>[4x]MAPTNESPKHAETRIVTDAPRNSESVGDHLFNGGVNHHDEDPDAYTKMYGPLVGYDPRNPTTLFANARQTGTQLVAPRKAREILTGIYSFEPTVLAFQREFVKRANAVAQPDLNSDGFSLNGLHTTFDSIRSVSGYPQWPVSALPKSNVGLLRDLKLQERMTARQVVIAREIWKRVWGHMKPTAIKIPKMSTSGPPRNVNDAEMKLQYALALFSGNRYNGYLDAFKSGDLSRFYRDYEAAVIMGTNVRWQVDNPGKKRDYWAQADIERELAPSKRPITTKVEINGTVYDDFAAMRTRLVNAGPWTINVALQPFATGCMNAMFELYRATWHPDEDKIAGFLEGKHAFFGDVSSY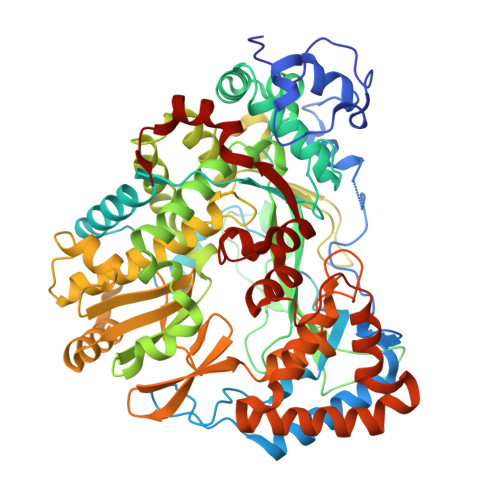DHSFSEEKIDLSLEVGKEFISPEIMELASSLFYAAYFTRPLGPDDGPQLVGNPNRYLEKQVKAGNRSGHAFTSLFAKVWKVIDTVSKFDQMGYDVVANMDAILKGDMPFGCINNGDDEIVWFKSERDYRLFLRLLETQPQEQRMFKVGPEEGAVFSGSVYQLIGPLKYQAVERITTPFQRIICPERSIGGNFRKFWPLGILERYNKRNSHPVLEEVWRVFDDTYATLMEPHYGSFLGIVQRAHKEIPFSVDDLSWKEIMVLDDPNKMYHRFTDEEIRDQVQESAFRKLQPIFFERMFKEHYKGNYV(2R)-7-amino-2-(sulfanylmethyl)heptanoic acid | C8 H17 N O2 S | 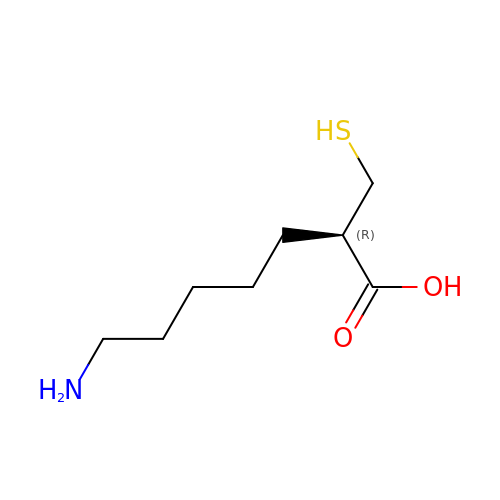OWVFNXQLXNWAHW-ZETCQYMHSA-N>MASKEEDNMASLPKTHELHIFGSFNGVKFDMVGEGTGNPNEGSEELKLKSTNGPLKFSPYILVPHLXFYQYLPFPDGMSPFQAAMHDGSGYQVHRTIQYEDGASVTAHYRYTYEGSHIKGEFQVIGTGFPPDGPVMTNKLTAMDWSVTKMLYPNDKTILSTADCSYTTTAGKRYQSKMRENNTFAKPMAADILQKQPMFVFRKSELQHSKTELTFKEWQKAFTDVMSG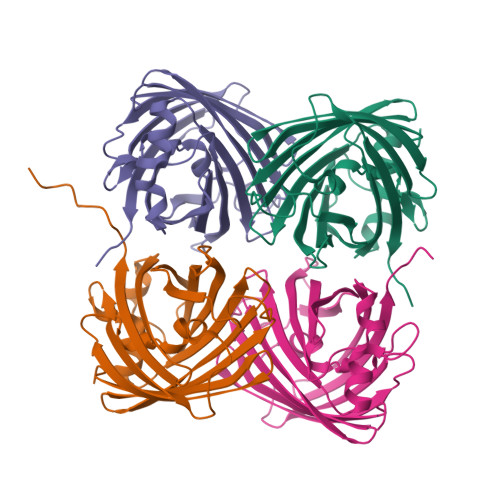GSHHHHHH[4x]>[12x]GSHMPKRTFTKEDIRKFAEEENVRYLRLQFTDILGTIKNVEVPVSQLEKVLDNEMMFDGSSIEGFVRIEESDMYLHPDLDTWVIFPWTAGQGKVARLICDVYKTDGTPFEGDPRANLKRVLKEMEDLGFTDFNLGPEPEFFLFKLDEKGEPTLELNDDGGYFDLAPTDLGENCRRDIVLELEDMGFDIEASHHEVAPGQHEIDFKYADAVTACDNIQTFKLVVKTIARKHNLHATFMPKPLFGVNGSGMHFNVSLFKGKENAFFDPNTEMGLTETAYQFTAGVLKNARGFTAVCNPLVNSYKRLVPGYEAPCYIAWSGKNRSPLIRVPSSRGLSTRIEVRSVDPAANPYMALAAILEAGLDGIKNKLKVPEPVNQNIYEMNREEREAVGIQDLPSTLYTALKAMRENEVIKKALGNHIYNQFINSKSIEWDYYRTQVSEWERDQYMKQY

In Gram-positive bacteria, nitrogen homeostasis is controlled by an operon encoding glutamine synthetase (GS), a dodecameric machine that assimilates ammonium into glutamine, and the GlnR repressor. GlnR detects nitrogen excess indirectly by binding glutamine-feedback-inhibited-GS (FBI-GS), which activates its transcription-repression function. GS generates glutamine from glutamate, ATP, and ammonium by a mechanism that involves the initial phosphorylation of the γ-carboxyl group of glutamate by ATP and the subsequent incorporation of ammonium. The structures show FBI-GS binds the GlnR C-terminal domain within its active-site cavity, juxtaposing two GlnR monomers to form a DNA-binding-competent GlnR dimer.

Thus, we next obtained cryo-EM structures of apo Pp, Lm, and Sa GS to resolutions of 3.16, 2.85, and 2.13 Å, respectively. These structures revealed that, like the Bs apo GS, the Lm, Sa, and most of the Pp apo GS states are dodecamers. Interestingly, overlays of the individual GS subunits show that the apo GS subunits are similar to those in the FBI-GS-GlnR complexes (rmsds of 0.5–0.8 Å for overlay of 400 corresponding Cα atoms between GS proteins). In this conformation, key active site residues are not properly positioned for catalysis. In particular, the Arg62 side chain is rotated into the active site preventing the proper positioning of the catalytic Asp50´ side chain and Arg316, which assists in catalysis, is moved out of the active site. Hence, conformational changes in the apo states would be needed to generate an enzymatically active conformation unless these enzymes employ a catalytic mechanism different from other GS. In fact, the electron density for the active site regions of the apo GS structures are poorly defined indicating flexibility in these regions. This suggests that they could undergo conformational changes during catalysis. Thus, our structural analyses indicate that GS enzymes from low G + C Gram-positive bacteria adopt two distinct states, the active, TS conformation (herein termed the “A” state) and the conformation adopted by apo GS/FBI-GS-GlnR, termed the “I” or inhibited state.>[2x]MPLTDTDRSEDFLRRVRGLKAARTANGPRLYQPITLLWAVGRARRGEARTLAWADTDEAIGALLKRHGARGERPRPDYPVLALHRAGLWTLEGHVGEVPTAHGDSALRNWFAEQRPVGGLAEPFHDLLHRSGHSRVSVIEALLTTYFAGLDPVPLLEDTGLYDEG

The sulfur atom of phosphorothioated DNA (PT-DNA) is coordinated by a surface cavity in the conserved sulfur-binding domain (SBD) of type IV restriction enzymes. The sulfur modification-dependent REases SprMcrA and ScoMcrA use an SBD to recognize the DNA backbone phosphorothioate link of the RP stereoisomer, which is adopted by the naturally occurring PT modifications in five DNA core sequence contexts in prokaryotes. By contrast, the SBD of the PT-dependent restriction endonuclease (REase) SprMcrA from Streptomyces pristinaespiralis has a relatively relaxed sequence specificity, targeting GPSGCC, GPSAAC and GPSATC, but not GPSTTC or CPSCA. The sulfur atom of the PT linkage was inserted into a cavity which formed by Y31, Q32, Y78, P79 and A82 through Van der Waals interactions; the phosphate groups flanking the PT linkage formed electrostatic bonds with R29, R73 and R85, as well as hydrogen bonds with Y31 and A101.

Crystals for SBDSpr in complex with the RP form of the 8-bp hemi-PT DNA oligonucleotide 5′-GATGPSATCC-3′ were grown at 14°C with the reservoir solution containing 0.1 M Tris–HCl pH 8.5 and 4.5% PEG 8000. The SBDSpr–GPSATC complex crystals belonged to the C2221 space group, with two molecules of SBDSpr and two molecules of GPSATC–DNA in the asymmetric unit; the structure of this complex was determined to 3.3 Å by the molecular replacement method with the Phaser program, using the structure of SBDSpr–GPSAAC as the searching model. SBDSpr showed the highest binding affinity for GPSGCC, with a dissociation constant value (KD) of 5.55 nM, followed by a KD of 38.33 nM for GPSATC and 94.67 nM for GPSAAC. In all structures, the ND1 atom of H102 formed H-bond with O6 atom of G4, and the OD2 atom of D104 bonded to the N4 atom of C7. It's worth noting that the ND1 atom of H102 also formed H-bond with N7 atom of G4 in GPSGCC and GPSAAC sequences, while this H-bond was not existing in SBDSpr-GPSATC complex. SA5 showed a significant deflection in GPSATC sequence, compared with GPSGCC and GPSAAC sequences, leading to formation of another H-bond between the ND1 atom of H102 with the N6 atom of SA5. In conclusion, HGD motif formed five H-bonds in SBDSpr–GPSGCC complex while four H-bonds in SBDSpr–GPSATC and SBDSpr–GPSAAC complexes, which explained why SBDSpr showed a highest affinity for GPSGCC. In the case of GPSATC, the percent solvent accessibility of T6 methyl group was calculated to be only 10–15, corresponding to fully buried with the SBD-DNA interface. The multiple C–H…O contacts between the methyl and Y78 were believed to be attractive for GPSATC. Difference in the weak non-bonded interaction between GPSATC and GPSAAC results in a lower KD values for GPSATC than GPSAAC bound by SBDSpr.> GSHMRNVAAEQQLRELESTFDGRLGFVALDTATGARIAHRADERFPFCSTFKTMLSAAVLARS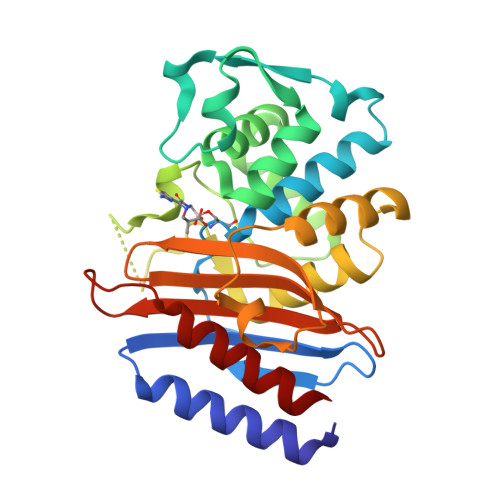AGDAALLQRRIPYAKRDLVRYSPITEKHVGAGMTVAELCAATLQYSDNTAANLLIALLGGPQAVTAYARSIGDATFRLDRRETELNTAIPGDERDTTTIPGDERDTTTPAAMAASVRRLLVGDALGTAQRAQLNAWMLGNKTGDARIRAGVPAGWRVADKTGTGDYGTGNDIGVAYPPDRAPIVFVVYTTMRSRNAQARDDVIASAARIAARAFV>[3x]MGASANALGMIETKGLVGAIEAADAMVKAANVQLVGKEQVGGGLVTVMVRGDVGAVKAATDAGAAAAERVGELISVHVIPRPHFEVDAILPKVSAELEHHHHHH

To understand the structure and function of the C. difficile eut bacterial microcompartment we have determined the crystal structures of two proteins with homology to BMC shell proteins, CD1908 and CD1918, and show that they are well conserved between species. We have also determined the atomic structure of CD1925, a member of the EutQ family of cupin barrels. The sequestration of ethanolamine metabolism within a BMC is thought to protect the cell from the acetaldehyde produced as an intermediate in its breakdown and to prevent the loss of this volatile compound and its carbon from the cell.

The structure of CD1918 was determined by molecular replacement to 1.62 Å. Three protein chains were present in the asymmetric unit, with each chain visible in electron density to residue ninety of the polymer. CD1918 displays the canonical BMC fold with a four-stranded anti-parallel β-sheet flanked by α-helices, and forms a hexamer with molecules related by a crystallographic 2-fold axis. The oligomer of CD1918 has much flatter faces than CD1908 and it has an open pore at its centre. The faces of CD1918 are primarily negatively charged, with positive patches around the sides of the hexamer and a positively charged pore. This pore is 9 Å in diameter and its boundary is demarcated by a loop between β-strands 1 and 2, with the amide nitrogen of Gly41 and the side-chain of Lys41 (Fig. 5E/F) forming the boundary of the pore. Electron density consistent with a sulphate molecule, a component of the crystallisation condition, was built within the pore, and there are a series of water molecules above and below the pore. The presence of a sulphate ion within this pore, and its narrow width, suggest that small polar, or charged, molecules would be the most probable candidate ligands for transport through the BMC shell by this protein. This protein may be a channel for water, or a conduit for the transport of the ethanolamine substrate, or for the exit of the acetyl-phosphate produced by the phosphotransacetylase encoded by CD1920.> AEYVRALFDFNGNDEEDLPFK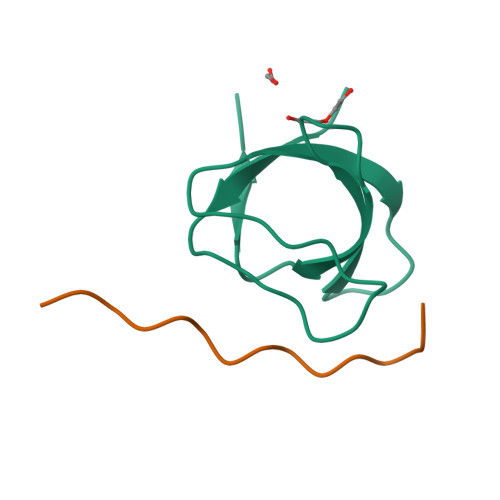KGDILRIRDKPEEQWWNAEDSEGKRGMIPVPYVEKYR;> XDNSPPPALPKKRQSYX2(S)-AMINO-6-BORONOHEXANOIC 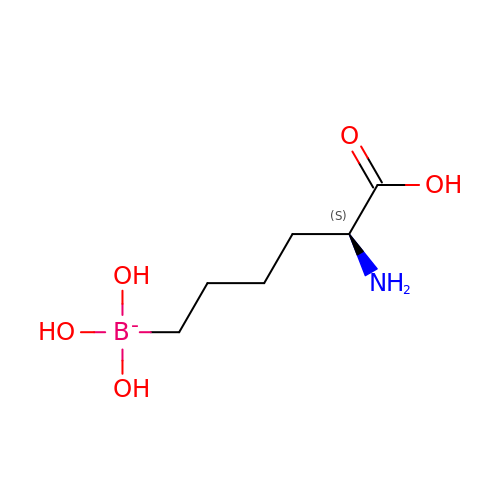ACID | C6 H15 B N O5 | BLVGFZFOWWBCCZ-YFKPBYRVSA-N> GSTSARNHTEDNSTEYYDYEEARCACPARHLNNTNGTVLKPLGCHY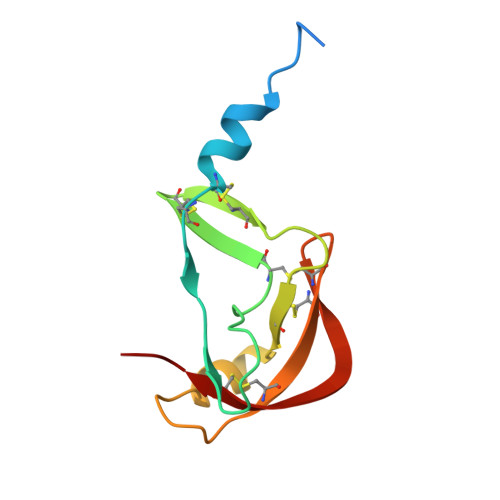FCNGTLCTAPDGYPCYNLTAQQVRTLTTYPNTSCAVGVCMKGTCVKNGTMEQCFKTP> MAETSEEVAVLVQRVVKDITNAFRRNPHIDEIGLIPCPEARYNRSPIVLVENKLGVESWCVKFLLPYVHNKLLLYRTRKQWLNRDELIDVTCTLLLLNPDFTTAWNVRKELILSGTLNPIKDLHLGKLALTKFPKSPETWIHRRWVLQQLIQETSLPSFVTKGNLGTIPTERAQRLIQEEMEVCGEAAGRYPSNYNAWSHRIWVLQHLAKLDVKILLDELSSTKHWASMHVSDHSGFHYRQFLLKSLISQTVIDSSVMEQNPLRSEPALVPPKDEEAAVSTE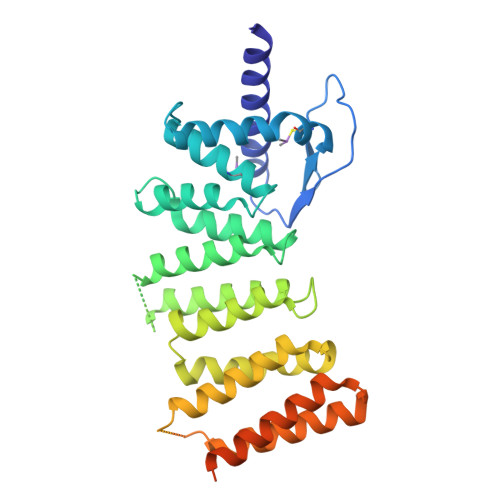EPRINLPHLLEEEVEFSTDLIDSYPGHETLWCHRRHIFYLQHHLNGRFPHSMTQLSPADSPGGTLSDLHLIPAGSQLSQAMEVD>MKHMPRKMYSCAFETTTKVEDCRVWAYGYMNIEDHSEYKIGNSLDEFMAWVLKVQADLYFHNLKFAGAFIINWLERNGFKWSADGLPNTYNTIISRMGQWYMIDICLGYKGKRKIHTVIYDSLKKLPFPVKKIAKDFKLTVLKGDIDYHKERPVGYKITPEEYAYIKNDIQIIAEALLIQFKQGLDRMTAGSDSLKGFKDIITTKKFKKVFPTLSLGLDKEVRYAYRGGFTWLNDRFKEKEIGEGMVFDVNSLYPAQMYSRLLPYGEPIVFEGKYVWDEDYPLHIQHIRCEFELKEGYIPTIQIKRSRFYKGNEYLKSSGGEIADLWLSNVDLELMKEHYDLYNVEYISGLKFKATTGLFKDFIDKWTYIKTTSEGAIKQLAKLMLNSLYGKFASNPDVTGKVPYLKENGALGFRLGEEETKDPVYTPMGVFITAWARYTTITAAQACYDRIIYCDTDSIHLTGTEIPDVIKDIVDPKKLGYWAHESTFKRAKYLRQKTYIQDIYMKEVDGK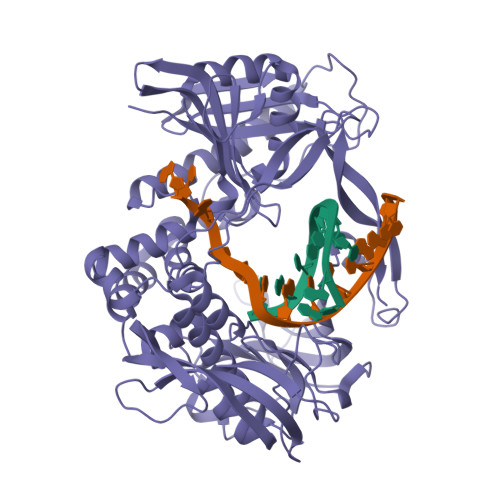LVEGSPDDYTDIKFSVKCAGMTDKIKKEVTFENFKVGFSRKMKPKPVQVPGGVVLVDDTFTIK[4x]>[3x]GPVVSIIRDDLTPQERERLMMRVRAALVDLGVAVGASVAFRQLTEPMKSEIA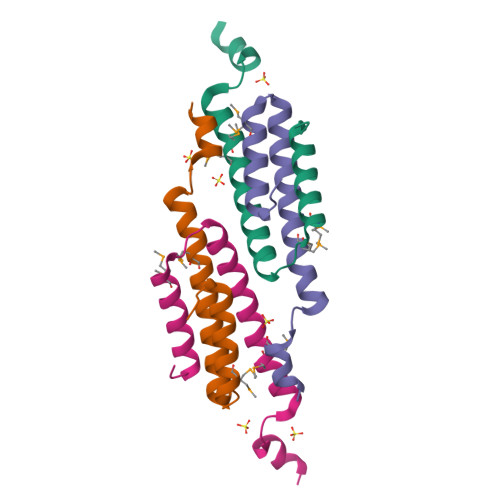ATVKKYLEYDH> MAPTAVCSDGTRVSNAVCCDFVSLGQDLQSMVLQGDCGEDAHEIIRLTFHDAVAISRKLGPSAGGGADGSMLLFPLVEPEFAASNGIDDSVNNLIPFLSLHPTISAGDLVQFAGAVALSNCPGAPRVQFLAGRPNHTIAAIDGLIPEPQDNVTSILERFDDAGGFTPFEVVSLLASHTIARA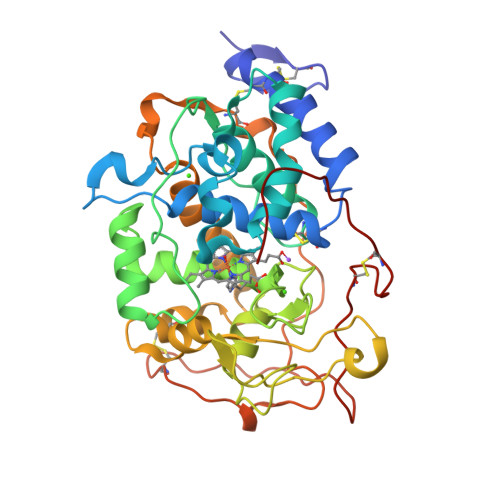DKVDPTLDAAPFDTTPFTFDSQIFLEVLLKGVGFPGLDNNTGEVSSPLPLGDTSTGGKDTGLMRLQSDFALAHDPRTACFWQGFVDQQEFMSQSFASAFAKLAVLGHNTDDLIDCSEVVPVPKPAVDKPTTFPATTGPQDLELSCLAERFPTLSVDPGAQETLIPHCSDGLENCTSVQFSGPATDSP2,4-DIOXO-PENTANEDIOIC 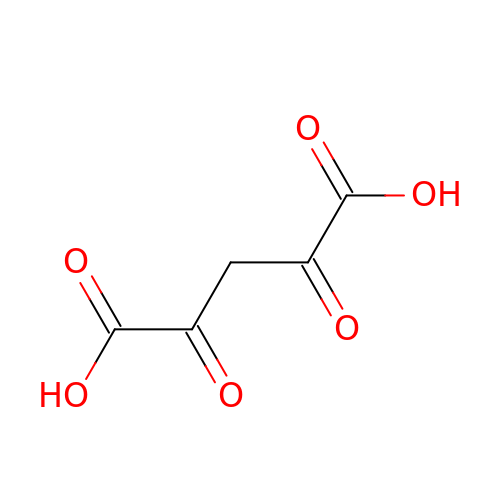ACID | C5 H4 O6 | TVKBBTQJNQDZRU-UHFFFAOYSA-N> SYDYMEGGDIRVRRLFCRTQWYLRIDKRGKVKGTQEMRNSYNIMEIRTVAVGIVAIKGVESEYYLAMNKEGKLYAKQTPNEECLFLERLEENHYNTYISKKHAEK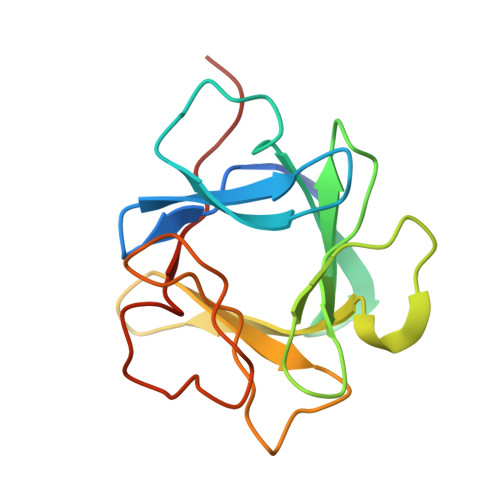NWFVGLKKNGSCKRGPRTHYGQKAILFLPLPVSSD2.5-anhydro-D-mannitol 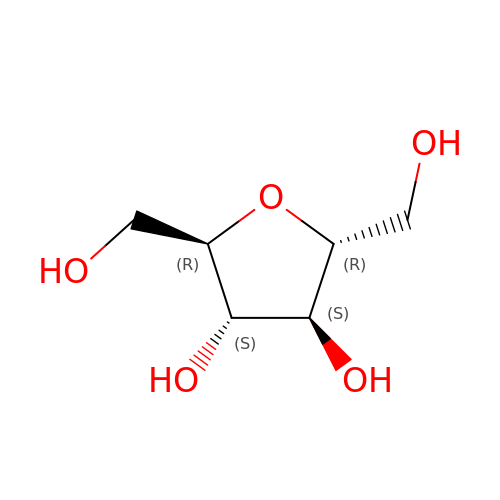| C6 H12 O5 | MCHWWJLLPNDHGL-KVTDHHQDSA-N>MHHHHHHDEKRENDPAKVKEAILAAKAAGRSRKDGNLERAMTI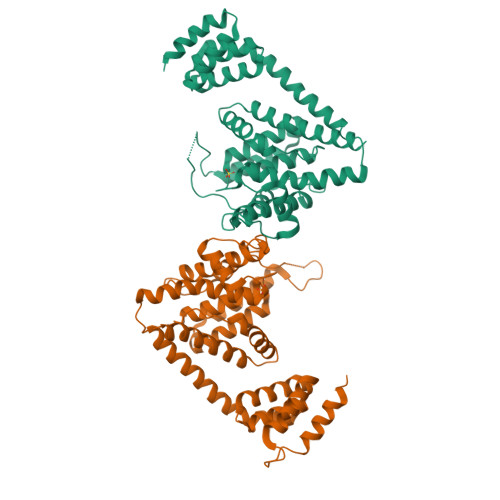MEHAMALAPTNPQILIEMGQIREMHNELVEADQCYVKALAYDPGNSEALVLRARTTPLVSAIDRKMLRSVHDLRDEFNHLQHSTALRRMMRETYFLYVYHTVAIEGNTLSLGQTRAILESGMVIPGKSIREHNEVIGMDAALRFLNCSLLSKEHDEISIDDILEMHRRVLGNADPVEAGRIRTTQVYVGRFTPVSPEYVMEQLKDIVDWLNDESTLTIDPIERAAIAHYKLVLVHPFTDGNGRTARLLLNLIMMRSGFPPVILPVETRAEYYASLHVANLGDLRPFVRYVAKHSEASIQRYIGAMKTSSDNILNSGDSKLTPEESEVSEKIEAECRAGN[2x]> XXXXXXXXXXXXXXXXXXXXXXXXXXXXXXXXXXXXXXXXXXXXXXXXXXXXXXXXXXXXXXXXXXXX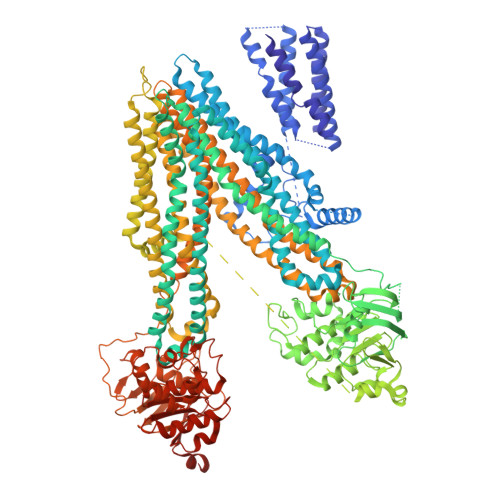XXXXXXXXXXXXXXXXXXXXXXXXXXXXXXXXXXXXXXXXXXXXXXXXXXXXXXXXXPNPCPESSASFLSRITFWWITGMMVQGYRQPLESTDLWSLNKEDTSEQVVPVLVKNWKKECAKSRKQPVKIVYSSKDPAKPKGSSKVDVNEEAEALIVKCPQKERDPSLFKVLYKTFGPYFLMSFLFKAVHDLMMFAGPEILKLLINFVNDKKAPEWQGYFYTALLFISACLQTLVLHQYFHICFVSGMRIKTAVIGAVYRKALVITNAARKSSTVGEIVNLMSVDAQRFMDLATYINMIWSAPLQVILALYLLWLNLGPSVLAGVAVMVLMVPLNAVMAMKTKTYQVAHMKSKDNRIKLMNEILNGIKVLKLYAWELAFKDKVLAIRQEELKVLKKSAYLAAVGTFTWVCTPFLVALSTFAVYVTVDENNILDAQKAFVSLALFNILRFPLNILPMVISSIVQASVSLKRLRVFLSHEDLDPDSIQRRPIKDAGATNSITVKNATFTWARNDPPTLHGITFSVPEGSLVAVVGQVGCGKSSLLSALLAEMDKVEGHVTVKGSVAYVPQQAWIQNISLRENILFGRQLQERYYKAVVEACALLPDLEILPSGDRTEIGEKGVNLSGGQKQRVSLARAVYCDSDVYLLDDPLSAVDAHVGKHIFENVIGPKGLLKNKTRLLVTHAISYLPQMDVIIVMSGGKISEMGSYQELLARDGAFAEFLRTYASAEQEQGQPEDGLAGVGGPGKEVKQMENGMLVTDTAGKQMQRQLSSSSSYSRDVSQHHTSTAELRKPGPTEETWKLVEADKAQTGQVKLSVYWDYMKAIGLFISFLSIFLFLCNHVASLVSNYWLSLWTDDPIVNGTQEHTQVRLSVYGALGISQGITVFGYSMAVSIGGIFASRRLHLDLLHNVLRSPISFFERTPSGNLVNRFSKELDTVDSMIPQVIKMFMGSLFNVIGACIIILLATPMAAVIIPPLGLIYFFVQRFYVASSRQLKRLESVSRSPVYSHFNETLLGVSVIRAFEEQERFIRQSDLKVDENQKAYYPSIVANRWLAVRLECVGNCIVLFASLFAVISRHSLSAGLVGLSVSYSLQVTTYLNWLVRMSSEMETNIVAVERLKEYSETEKEAPWQIQDMAPPKDWPQVGRVEFRDYGLRYREDLDLVLKHINVTIDGGEKVGIVGRTGAGKSSLTLGLFRIKESAEGEIIIDDINIAKIGLHDLRFKITIIPQDPVLFSGSLRMNLDPFSQYSDEEVWTSLELAHLKGFVSALPDKLNHECAEGGENLSVGQRQLVCLARALLRKTKILVLDEATAAVDLETDDLIQSTIRTQFDDCTVLTIAHRLNTIMDYTRVIVLDKGEIQEWGSPSDLLQQRGLFYSMAKDSGLVSNSLEVLFQ>[2x]MGSSHHHHHHSQDP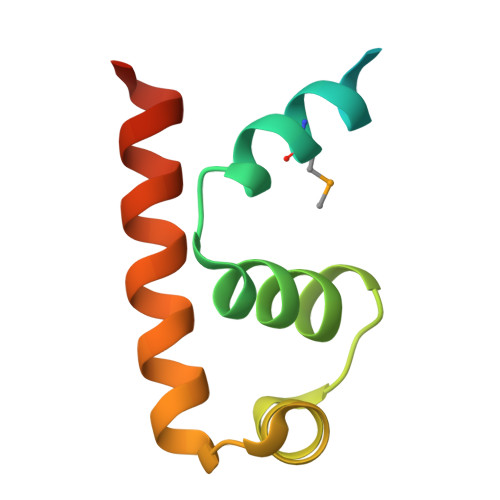MAIEADSVTRMNELLEILPAKQREILILRVVVGLSAEETAAAVGSTTGAVRVAQHRALQRLKDEIVAAGDYA> GSEAAGGEQRELLIQRLRAAVHYTTGALAQDVAE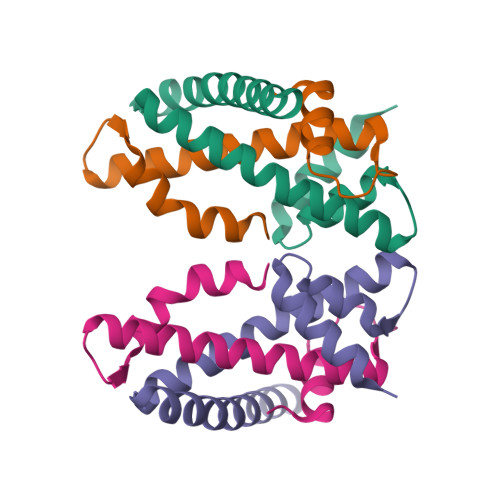DKGVLFSKQTVAAISEITFRQAENFARDLEMFARHAKRSTITSEDVKLLARRSNSLLKYITQKSDELASSNME;> GYEEREGGFRKETVERLLRLHFRDGRTRVNGDALLLMAELLKVFVREAAARAARQAQAEDLEKVDIEHVEKVLPQLLLDFV>MKEFYLTVEQIGDSIFERYIDSNGRERTREVEYKPSLFAHCPESQATKYFDIYGKPCTRKLFANMRDASQWIKRMEDIGLEALGMDDFKLAYLSDTYNYEIKYDHTKIRVANFDIEVTSPDGFPEPSQAKHPIDAITHYDSIDDRFYVFDLLNSPYGNVEEWSIEIAAKLQEQGGDEVPSEIIDKIIYMPFDNEKELLMEYLNFWQQKTPVILTGWNVESFDIPYVYNRIKNIFGESTAKRLSPHRKTRVKVIENMYGSREIITLFGISVLDYIDLYKKFSFTNQPSYSLDYISEFELNVGKLKYDGPISKLRESNHQRYISYNIID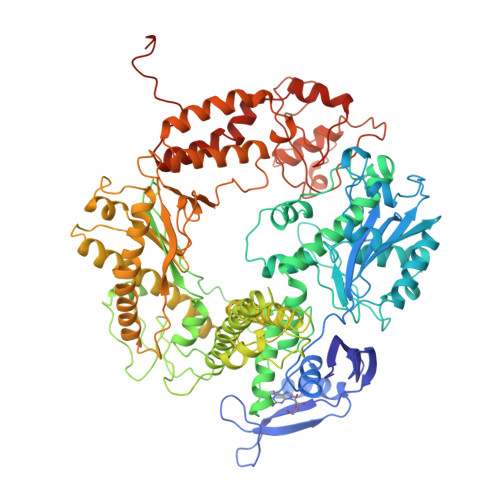VYRVLQIDAKRQFINLSLDMGYYAKIQIQSVFSPIKTWDAIIFNSLKEQNKVIPQGRSHPVQPYPGAFVKEPIPNRYKYVMSFDLTSLYPSIIRQVNISPETIAGTFKVAPLHDYINAVAERPSDVYSCSPNGMMYYKDRDGVVPTEITKVFNQRKEHKGYMLAAQRNGEIIKEALHNPNLSVDEPLDVDYRFDFSDEIKEKIKKLSAKSLNEMLFRAQRTEVAGMTAQINRKLLINSLYGALGNVWFRYYDLRNATAITTFGQMALQWIERKVNEYLNEVCGTEGEAFVLYGDTDSIYVSADKIIDKVGESKFRDTNHWVDFLDKFARERMEPAIDRGFREMCEYMNNKQHLMFMDREAIAGPPLGSKGIGGFWTGKKRYALNVWDMEGTRYAEPKLKIMGLETQKSSTPKAVQKALKECIRRMLQEGEESLQEYFKEFEKEFRQLNYISIASVSSANNIAKYDVGGFPGPKCPFHIRGILTYNRAIKGNIDAPQVVEGEKVYVLPLREGNPFGDKCIAWPSGTEITDLIKDDVLHWMDYTVLLEKTFIKPLEGFTSAAKLDYEKKASLFDMFDF[2x]> AF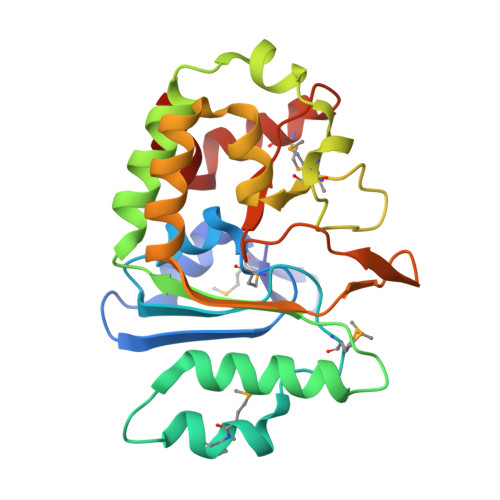GQDGNNWMEIDDLAKGLPDDLFDFILFDACYMASVECTYELRNKAEYILASPTETMADGWPYEEMMPQLFATDLQLEKVGETFYNHYLNNTYPYATVSLTKTSELDNLKSAIHDILADKTESDIYSLDPKNMQRLEYLYRSPGMLYDFNDYIKQLATAEQYDRFISCLDKAVVYKAHTPKSYYAAIGNALPIKSYCGLTIFVPQESLPKMLEWYKQRVGWYKAVYE> PS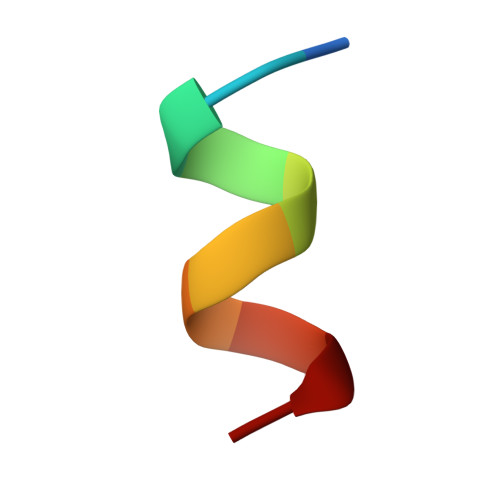ILKKILLE> MDAKKVAKKAADQAANRIRELAQVLVELLKEALKLDLTQEMRKKLIERYAAAIIRAIGDINNAIYQAKQEAEKLKKAGLVDSDQLDALLRALDELQK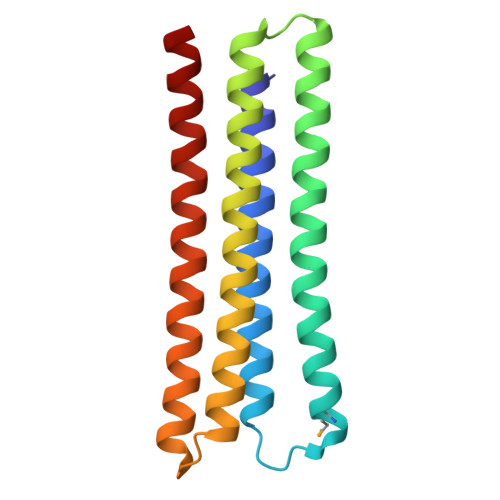VASKAANQLGRLFEEALKRLDKDNGGEEEKDRTAKWFEFEARAIAIALTLAAIGDVFDLEKEWRKLK>[2x]GMTKPKEPTALDLPMADPLPDETQKYFEICQEKLGMVPNVLKAYAFNVEKLNA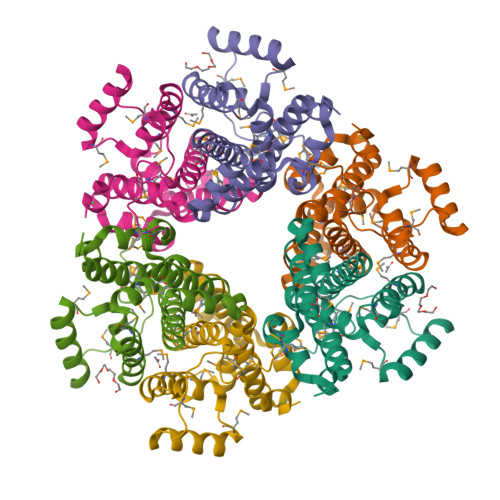FTAMYNDLMLGESQLSKLEREMIAVVVSSINKCFYCLVAHGAAVRQLSGDPQLGEMLVMNYRVAPLDARQRVMLDFAAKMTRASAEIEEADREVLRSHGFNDRDIWDIANVTGFFNMTNRVASATAMMPNAEYHGQFR> MGLQARSHSQARLDNLLNQELPAQVKGLAAHINLSLSQDL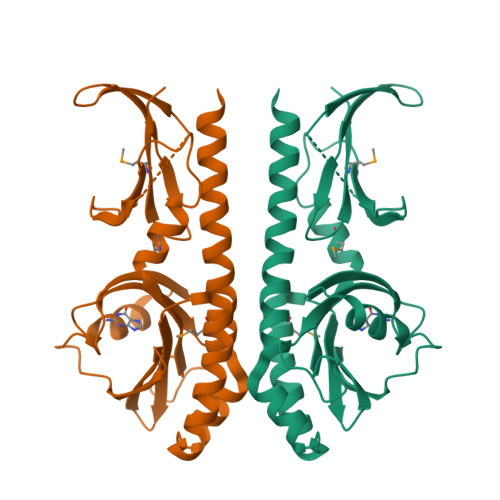AISESLANSYFIEQWVREGLPEERQNDIAAYLARLMEQLDTELLFIAAQHQGRGYYFQLRNGEFLQRIIQPPGSEDDWYYHFTDSDNAYELNLDSDTFSPDDAFVYVNYRSTVNAANGRPLVVAGAGLDLSQMASLIDDFRLGGSGHASLLSAEGELLVRSGEAKRSDESAPTVATATEALPEQASQRLLQNEQLQVHEATRDGQEVLVSTIWLPELQRYLMVEVDKKAYLASTHERFLELEHHHHHH>[2x]AIATSCHIAEEHIQKVAIFGGTHGNELTGVFLVKHWLENGAEIQRTGLEVKPFITNPRAVKKCTRYIDCDLNRIFDLENLGKKMSEDLPYEVRRAQEINHLFGPKDSEDSYDIIFDLHNTTSNMGCTLILEDSRNNFLIQMFHYIKTSLAPLPCYVYLIEHPSLKYATTRSIAKYPVGIEVGPQPQGVLRADILDQMRKMIKHALDFIHHF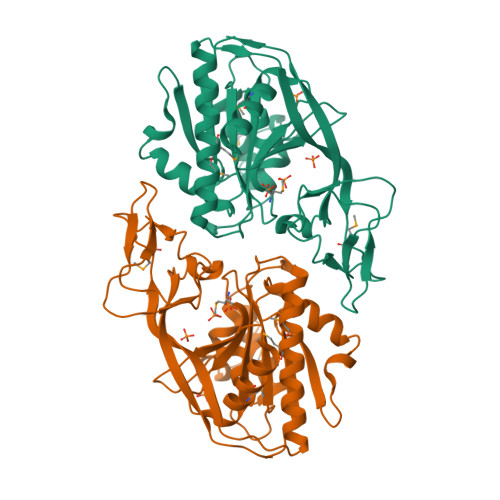NEGKEFPPCAIEVYKIIEKVDYPRDENGEIAAIIHPNLQDQDWKPLHPGDPMFLTLDGKTIPLGGDCTVYPVFVNEAAYYEKKEAFAKTTKLTLNAKSIRCCLH> MGSVWFRNRYWWYRSLYDDYVAREAKLAFGIAAFIWL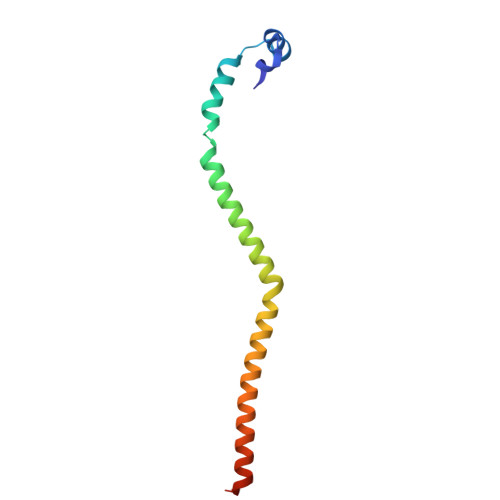PHYYWGIHLNRAFEVNFSHRNYAHEWGPRRNRLAHSLEFEQFDMILENWQDLEDEYAQRGDGMLKK5-FLUOROLEVULINIC ACID | C5 H7 F O3 | 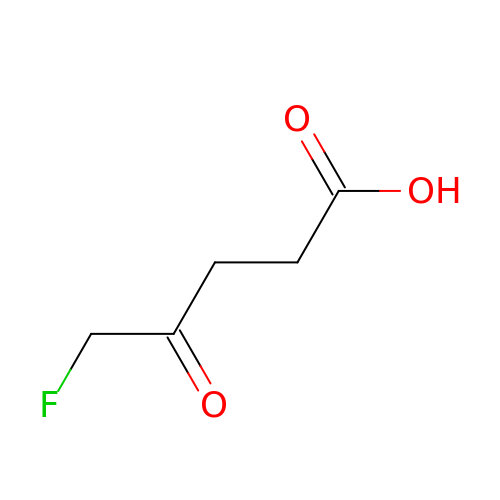MBVLGMJBSFUHKW-UHFFFAOYSA-N>MIIVTNTAKITKGNGHKLIERFNKVGKVETMPGFLGLEVLLTQNTVDYDEVTISTRWNAKEDFQGWTKSAAFKDAHSHQGGMPEYILDNKIAYYDVKVVRMPMAAAQ[2x]

Bacillus cereus (Bc) encodes three FNR paralogs, two of which have assigned distinct biological functions in bacillithiol disulfide reduction and flavodoxin (Fld) reduction. In this study, we have assigned a function to FNR1, in which the His residue is replaced by a conserved Val, in the reduction of the heme-degrading monooxygenase IsdG, ultimately facilitating the release of iron in an important iron acquisition pathway. The Bc IsdG structure was solved, and IsdG-FNR1 interactions were proposed through protein–protein docking. Mutational studies and bioinformatics analyses confirmed the importance of the conserved FAD-stacking residues on the respective reaction rates, proposing a division of FNRs into four functionally unique sequence similarity clusters likely related to the nature of this residue.

The IsdG monomers consist of Fd-like α/β-sandwich folds forming a β-barrel at the dimeric interface containing the conserved Asn-Trp-His triad required for the catalytic activity in the heme binding pockets. Bc IsdG was crystallized in its apo-form and reconstituted with hemin, the latter yielding red-brownish crystals. In this study, we demonstrate that the reduction of IsdG and IsdG-dependent heme degradation can be catalyzed by FNR1, as seen from our spectroscopic investigations after the addition of enzyme to a reaction mixture containing IsdG and NADPH. The reaction between FNR1 and IsdG proceeds with a kcat of 2.6 ± 0.2 min−1, the KM of FNR1 for IsdG was determined to be 2.1 ± 0.4 μM, and the catalytic efficiency (kcat/KM) was 1.2 ± 0.2 μM−1min−1. As we have demonstrated that FNR1 can reduce IsdG, the putative interaction was investigated through protein–protein docking. The selected top hits with the shortest heme-Fe (IsdG) to FAD-N5 (FNR) distances cover a large potential binding area of FNR1. In contrast to our previous docking results for Fld to FNR1 and FNR2, it seems likely that IsdG can bind in the less exposed binding cleft found in the FNR1 structure, which is narrower than the more “open” conformation observed in the FNR2 structure, with the latter suggested to facilitate binding of Fld. The docking of IsdG to multiple FNR1 sites, spreading across the binding site in a fan-like distribution, is in accordance with the interaction between cytochromes and methylamine dehydrogenase, where only an approximate orientation was needed for electron transfer.(2S)-1-(2,3-dihydro-1H-inden-2-ylamino)-3-(3,4-dimethylphenoxy)propan-2-ol | C20 H25 N O2 | 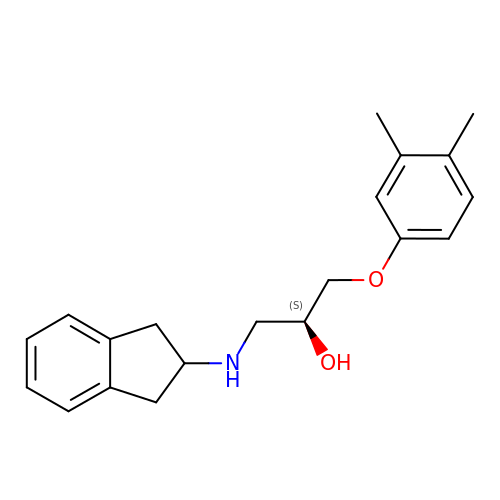ZDNVKJORSKCXID-IBGZPJMESA-N>[3x]IQKHKTLPKMSGGWELELNGTEAKLVRKVAGEKITVTFNINNSIPPTFDGEEEPSQGQKVEEQEPELTSTPNFVVEVIKNDDGKKALVLD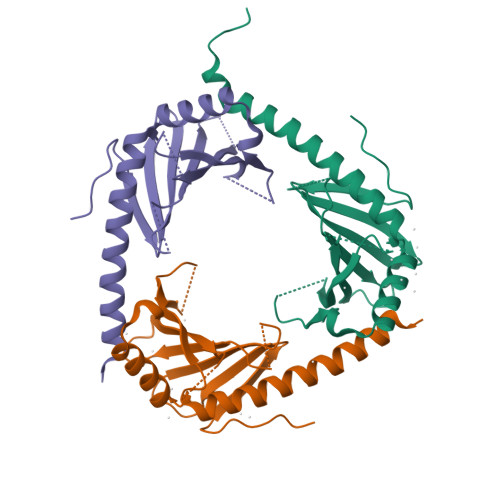CHYPEDEVGQEDEAESDIFSIREVSFQSTGESEWKDTNYTLNTDSLDWALYDHLMDFLADRGVDNTFADELVELSTALEHQEYITFLEDLKSFVKSQAHHHHHH>MTKLILIRAGETEWNLLGKIQGCTDIELTPNGIQQANEVAQQIKGNFDIIYSSPLHRALITAQKIAGDKEVHLIEGMKEIPFGTWEGHTFEELNGDINYKKFLSGEDGCPFDSTGMSIASWSKKNAQLLLDLCKQNENKTIVCVSHGAWIK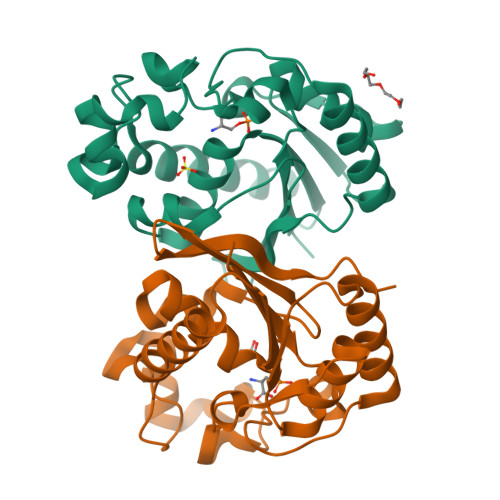TSILGLLEMEPTMYHKFQLGNTGITTFIFRHGHPVLTSFNSTQHLLTENKSKTGHHHHHH[4x]[(1-{2[(4-CARBAMIMIDOYL-PHENYLAMINO)-METHYL]-1-METHYL-1H-BENZOIMIDAZOL-5-YL}-CYCLOPROPYL)-PYRIDIN-2-YL-METHYLENEAMINOOXY]-ACETIC ACID ETHYL ESTER | C29 H31 N7 O3 | 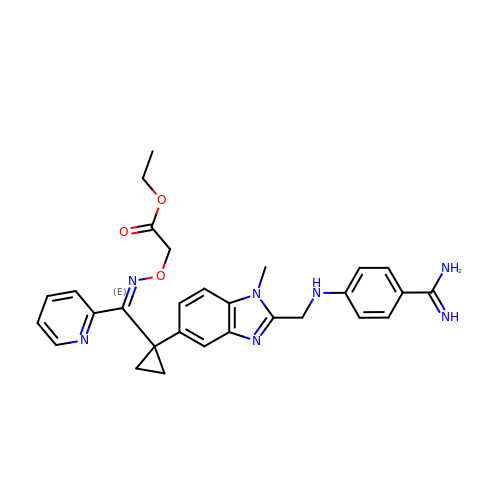RNOYCNIZOAIUSV-LSWMGQQCSA-N> SDAERRLAGLERASGARLGVYAYDTGSGRTVAYRADELFPMCSVFKTLSSAAVLRDLDRNGEFLSRRILYTQDDVEQADGAPETGKPQNLANGMTVEELCEVSITASDNCAANLMLRELGGPAAVTRFVRSLGDRVTRLDRWEPELNSAEPGRVTDTTSPRAITRTYGRLVLGDALNPRDRRLLTSWLLA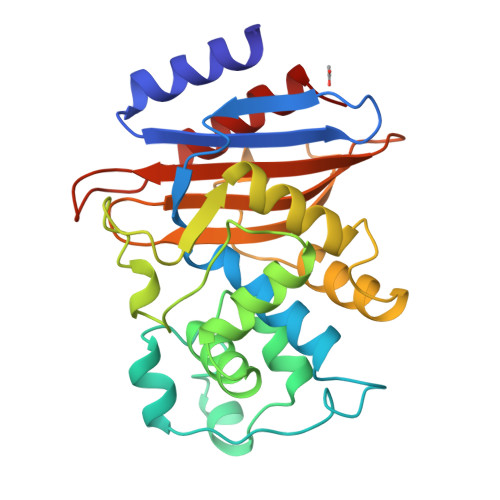NTTSGDRFRAGLPDDWTLGDKTGAGRYGTNNDAGVTWPPGRAPIVLTVLTAKTEQDAARDDGLVADAARVLAETLG>[2x]MQKQRTTSQWRELDAAHHLHPFTDTASL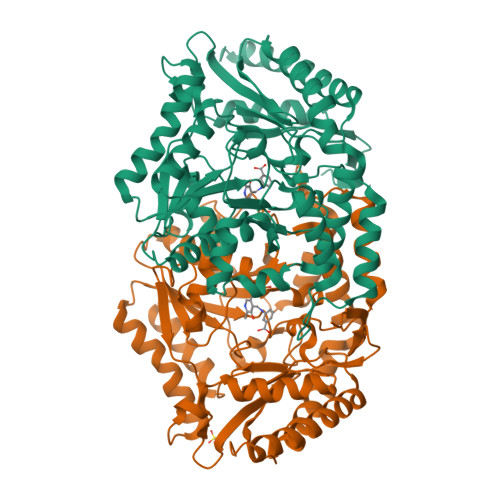NQAGARVMTRGEGVYLWDSEGNKIIDGMAGLWCVNVGYGRKDFAEAARRQMEELPFYNTFFKTTHPAVVELSSLLAEVTPAGFDRVFYTNSGSESVDTMIRMVRRYWDVQGKPEKKTLIGRWNGYHGSTIGGASLGGMKYMHEQGDLPIPGMAHIEQPWWYKHGKDMTPDEFGVVAARWLEEKILEIGADKVAAFVGEPIQGAGGVIVPPATYWPEIERICRKYDVLLVADEVICGFGRTGEWFGHQHFGFQPDLFTAAKGLSSGYLPIGAVFVGKRVAEGLIAGGDFNHGFTYSGHPVCAAVAHANVAALRDEGIVQRVKDDIGPYMQKRWRETFSRFEHVDDVRGVGMVQAFTLVKNKAKRELFPDFGEIGTLCRDIFFRNNLIMRACGDHIVSAPPLVMTRAEVDEMLAVAERCLEEFEQTLKARGLA>[2x]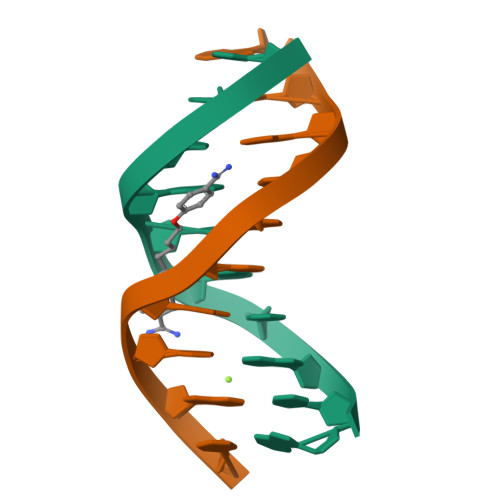ATATATATAT>GPPGPPGPPGP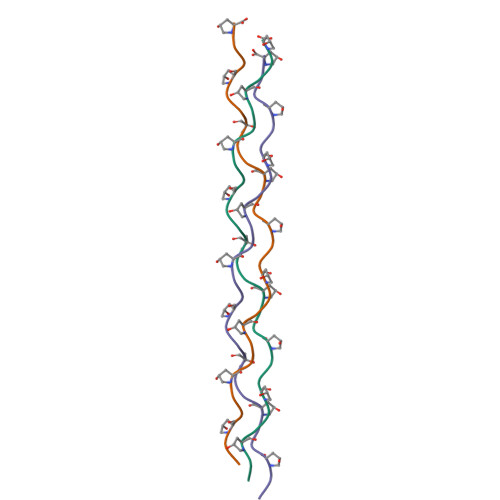PGPPGPPGPPGPPGPP[6x]> PTHIAIGILYKRGETPLPLVTFKYTDAQVQTVRKIAEEEGVPILQRIPLARALYWDALV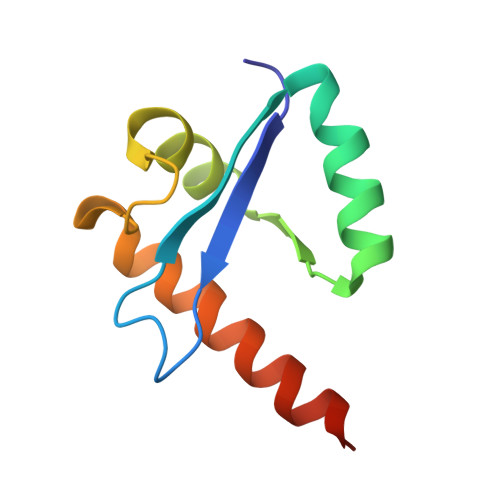DHYIPAEQIEATAEVLRWLERQNIEKQHSEML>MLLLTPGPTPIPERVQKALLRPMRGHLDPEVLRVNRAIQERLAALFDPGEGALVAALAGSGSLGMEAGLANLDRGPVLVLVNGAFSQRVAEMAALHGLDPEVLDFPPGEPVDPEAVARALKRRRYRMVALVHGETSTGVLNPAEAIGALAKEAGALFFLDAVTTLGMLPFSMRAMGVDYAFTGSQKCLSAPPGLAPIAASLEARKAFTGKRGWYLDLARVAEHWERGGYHHTTPVLLHYALLEALDLVLEEGVAARERRAREVYAWVLEELKARGFRPYPKASPLPTVLVVRPPEGVDADRLVRALYAEGVAVAGGIGPTR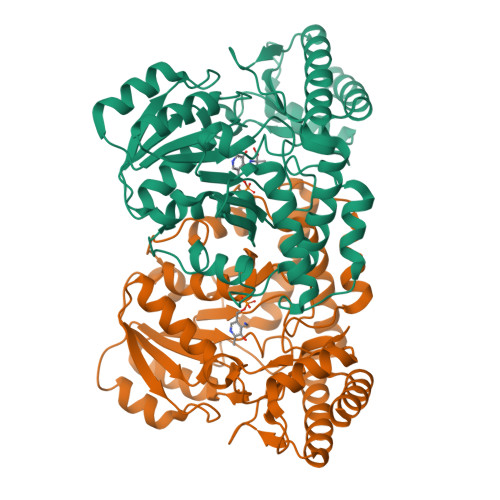GQVLRLGLMGEGARREAYQAFLKALDRALALA[2x]> ATSDSNMLL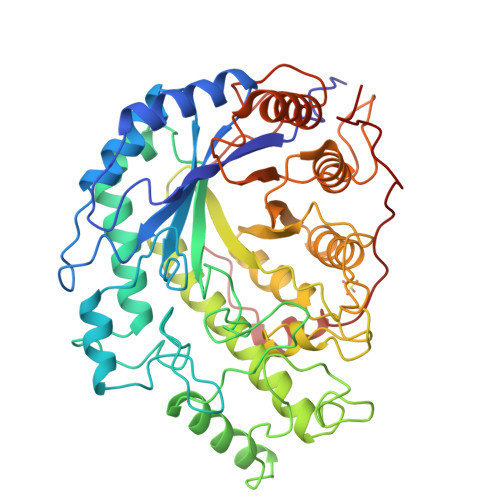NYVPVYVMLPLGVVNVDNVFEDPDGLKEQLLQLRAAGVDGVMVDVWWGIIELKGPKQYDWRAYRSLFQLVQECGLTLQAIMSFHQCGGNVGDIVNIPIPQWVLDIGESNHDIFYTNRSGTRNKEYLTVGVDNEPIFHGRTAIEIYSDYMKSFRENMSDFLESGLIIDIEVGLGPAGELRYPSYPQSQGWEFPRIGEFQCYDKYLKADFKAAVARAGHPEWELPDDAGKYNDVPESTGFFKSNGTYVTEKGKFFLTWYSNKLLNHGDQILDEANKAFLGCKVKLAIKVSGIHWWYKVENHAAELTAGYYNLNDRDGYRPIARMLSRHHAILNFTCLEMRDSEQPSDAKSGPQELVQQVLSGGWREDIRVAGENALPRYDATAYNQIILNAKPQGVNNNGPPKLSMFGVTYLRLSDDLLQKSNFNIFKKFVLKMHADQDYCANPQKYNHAITPLKPSAPKIPIEVLLEATKPTLPFPWLPETDMKVDG>GSHMNDVLVDAYNIAKDSQHVHGVHYIRGRNVGEDVHLAINIYVDADLKVFESDLVADAIRRKIEAEVDHVRDVHVGVT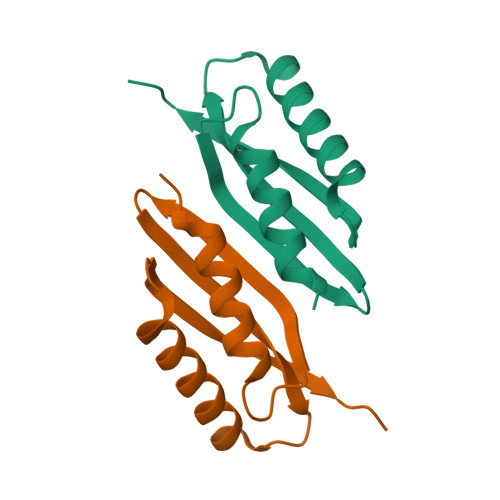PVRIAA[4x]> MGGKWSKSSIVGWPAIRERLRRAQPAAERRRAQPAAEGVGAASQDLGRHGALTSSNTDTTNADEEEEVGFPVRPQVPLRPMTYKGAVDLSFFLKEKGGLEGLVYSQREKEILDLWVYHTQGYFPDWQCYTPGPGVRYPLTFGWCFKLVPVDPGEVEEATEGENNC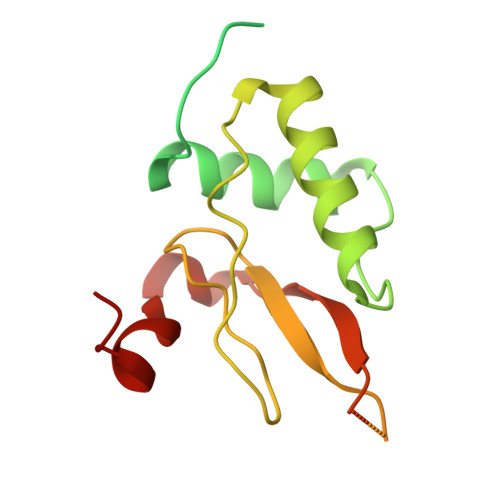LLHPICQHGMDDDHREVLKWKFDSHLAHTHMARELHPEYFKNC>[2x]MDLLSCTVNDAE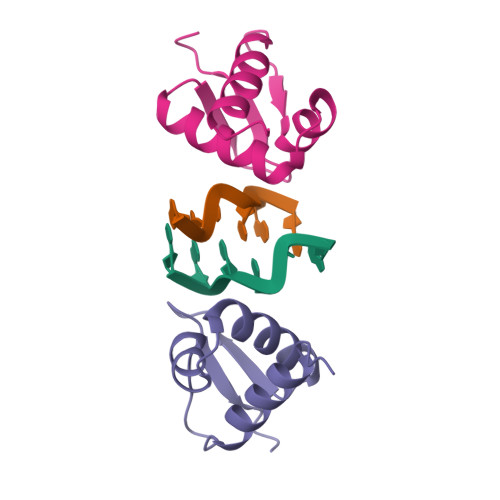IFSLVKKEVLSLNTNDYTTAISLSNRLKINKKKINQQLYKLQKEDTVKMVPSNPPKWFKNYNC>GPLGSSRLYLQNTAVMEELYRRNLSEDLVRDNGLSCGGREYWREPASTVGAASDGLSEEERRTAADAAERMTAVIAGTPGIAVERNVRDFRRGGWDVTPDNVESEFREVERRTFSDGVHWGRVIAFLAFSMSFAAY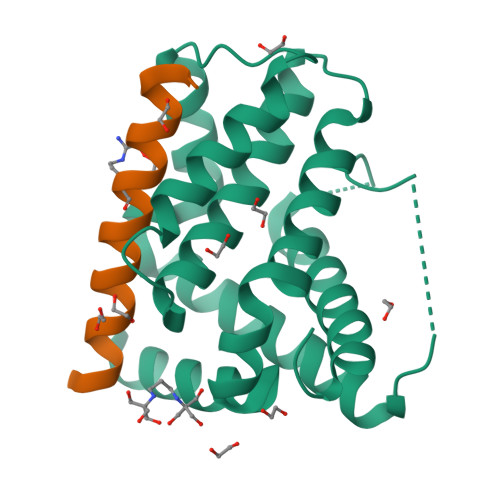VNSRGIDGGAYSVFNWTLRVLNDSLADFIQRENGWRGFIVYADTLLRAQGS[2x];>[2x]ASSMASEVGRRLAEFGDQVDGQFYQ4-NITRO-INDEN-1-ONE 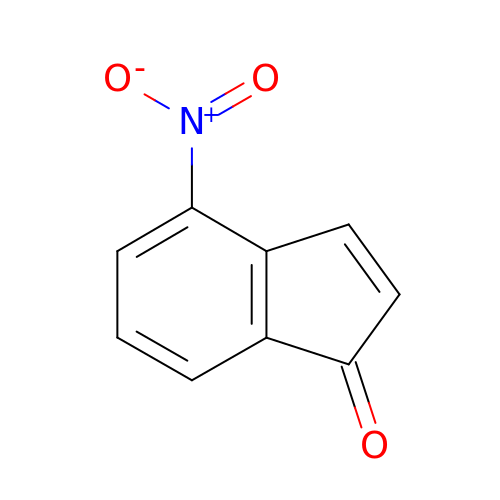| C9 H5 N O3 | UUNZJPCKMDLQPO-UHFFFAOYSA-N> GAMDPMATGDLKRSLRNLEQVLRLLNYPEEVDCVGLIKGDPAASLPIISYSFTSYSPYVTELIMESNVELIAKNDLRFIDAVYKLLRDQFNYKPILTKKQFIQCGFAEWKIQIVCDILNCVMKKHKELSSLQKIPSQQRKKISSG

CEP192 and CEP44 are proteins with a key role in centrosome and centriole biogenesis. We have recently determined the structures of the N-terminal Calponin Homology (CH) domain of human CEP44 and the so-called Spd2 domain of human CEP192. Both structures were obtained through X-ray crystallography at a resolution of 2.3 and 2.1 Å, respectively, and were experimentally phased. The N-terminal domain of CEP44 shares a weak sequence similarity to various CH domains, most of which members of the IFT81/NDC80/Hec families, whereas the Spd2 domain retrieves sequence matches to members of the PapD-like superfamily.

CEP44 was recently identified as a luminal centriolar protein that binds to the A-microtubules (MTs) of centrioles, as well as to the inner centriole protein POC1B20. The crystal structure of the CEP44 CH domain showed a typical CH fold consisting of a central four helical bundle elaborated with three short helices. The comparison of the experimental with the AF2 predicted structure (AF-Q9C0F1-F1-model_v1) revealed 116 residues superposed with rmsd of 0.74 Å. In contrast, the CEP44 experimental structure superposed with related CH domains with rmsd ranging from 2.8 to 3.1 Å. Thus, the AF2-predicted model is more similar to the experimental structure than any of the homologous templates available in the PDB. The predicted AF2 model has very similar or nearly identical backbone and side-chain conformations and is of comparable quality to the experimental crystal structure. The CEP44 CH-domain structure revealed the presence of a highly conserved basic patch on its surface. Mutation of the residues that constitute this patch abolish the CEP44 microtubule and centriole association, rationalising their involvement in microtubule binding. Even in the absence of the experimental CH-domain structure, the AF2 prediction model of this quality could be successfully used in cryo-EM-based microtubule docking studies or for further mutagenesis design aimed at the identification of additional CEP44 interaction partners. Besides the accurate prediction of the CEP44 N-terminal domain, the AF2 prediction of the alternating coiled coil and unstructured regions that follow the CH domain is in good agreement with other prediction methods and provides an easily accessible model of CEP44’s overall domain organisation.>SMADITTAEYHRLADEYLDALLSRLEELQDEREDVDVEYQSGVLTLNMGPEVGTYVINKQPPNKQIWLSSPKSGPKRYDYVITGEGQNEKQDTAVGEWVYLRDGSTLNQLLLEEIGVDLNVPVS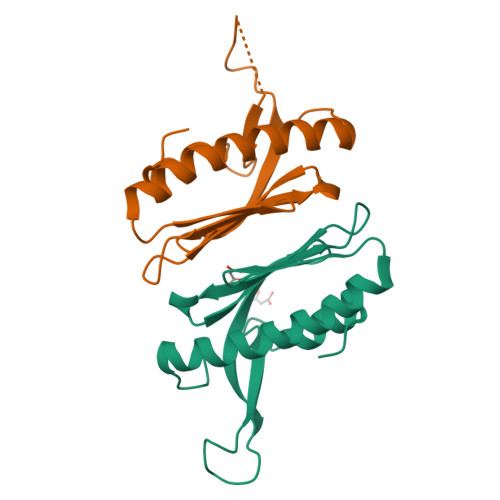QD[6x]>[2x]SNAMERKISDEECPVRK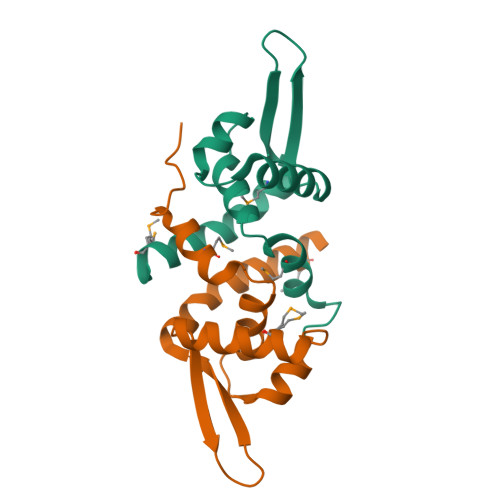SMQIFAGKWTLLIIFQINRRIIRYGELKRAIPGISEKMLIDELKFLCGKGLIKKKQYPEVPPRVEYSLTPLGEKVLPIIDEIAKFGMENL> GPAMKTLKDSKKLVRPQITDPYNPIVENANCPDINPIVAEYVLGNPTNVDAQLLDAVIFAFAEIDQSGNLFIPYPRFLNQLLALKGEKPSLKVIVAIGGWGAEGFSDAALTPTSRYNFARQVNQMINEYALDGIDIDWEYPGSSASGITSRPQDRENFTLLLTAIRDVIGDDKWLSVAGTG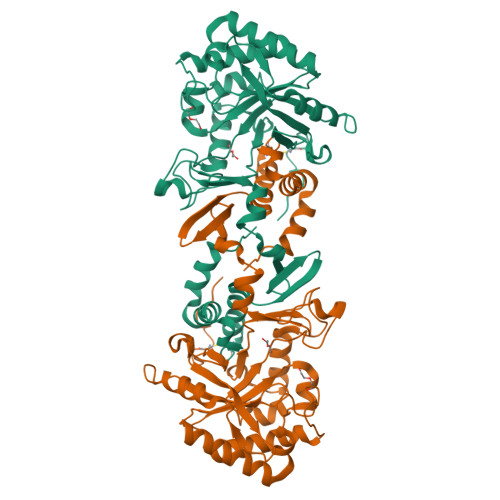DRGYINSSAEIDKIAPIIDYFNLMSYDFTAGETGPNGRKHQANLFDSDLSLPGYSVDAMVRNLENAGMPSEKILLGIPFYGRLGATITRTYDELRRDYINKNGYEYRFDNTAQVPYLVKDGDFAMSYDDALSIFLKTQYVLRNCLGGVFSWTSTYDQANILARTMSIGINDPEVLKEELEGIYGQF>[2x]HPICEVSKVASHLEVNCDKRQLTALPPDLPKDTTILHLSENLLYTFSLATLMPYTRLTQLNLDRCELTKLQVDGTLPVLGTLDLSHNQLQSLPLLGQTLPALTVLDVSFNRLTSLPLGALRGLGELQELYLKGNELKTLPPGLLTPTPKLEKLSLANNQLTELPAGLLNGLENLDTLLLQEN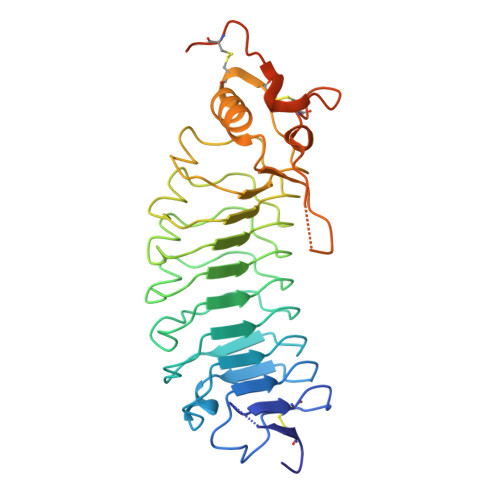SLYTIPKGFFGSHLLPFAFLHGNPWLCNCEILYFRRWLQDNAENVYVWKQGVDVKAMTSNVASVQCDNSDKFPVYKYPGKGCPTLGDEGDTDLYDYYPEEDTEGDKVR While the composition of MT nucleation systems is to some extent heterogeneous across eukaryotic organisms, γ-tubulin, a member of the tubulin superfamily, is a universal determinant in this process. In Saccharomyces cerevisiae, Spindle Pole body Component 97 (Spc97) and Spc98 were identified to assemble with two molecules of yeast γ-tubulin (Tub4) into the 300-kDa heterotetrameric γ-tubulin small complex (γ-TuSC), forming the core of the MT nucleation system in lower eukaryotes. The γ-TuSC possesses a Y-like overall shape of 180 Å height and a width of 60-100 Å. It is composed of two interacting spokes, each comprising one copy of γ-tubulin and either one molecule of Spc97 or Spc98. The N-terminal GRIP1 domain mediates canonical interactions between the Spc subunits, while the C-terminal GRIP2 domain binds one copy of γ-tubulin.

We isolated recombinantly expressed C. albicans γ-TuSC from insect cells by affinity purification and anion-exchange chromatography and used cryo-EM single particle analysis to obtain a structure at near-atomic resolution. We thus divided the γ-TuSC into two individual segments, each comprising one Spc protein and one γ-tubulin molecule, and refined them separately. This approach increased global resolution to 3.6 Å and improved density quality towards the periphery of the complex. Visual inspection of overlap, cross-correlation between density segments, and root mean square deviation (R.M.S.D) of protein backbone atoms in the atomic models consistently indicate that both copies of γ-tubulin in our cryo-EM reconstruction adopt a ‘straight’ conformation, as typically observed for αβ-tubulin dimers in stable and ordered microtubules. Thus, γ-tubulins in the fungal γ-TuSC are in a conformation that can promote growth of ‘straight’ microtubule protofilaments without a conformational change. Our cryo-EM density of the C. albicans γ-TuSC indicates binding of GDP, rather than GTP, and it remains to be addressed whether a nucleotide exchange to GTP is required to promote microtubule nucleation activity as suggested by analysis of γ-tubulin mutants in S. cerevisiae. In C. albicans, the first cluster of interactions is mostly formed by hydrophobic interactions between the GRIP1 domains of Spc97 and Spc98. In particular, the long insertion in the Spc98 GRIP2 domain (Asn626-Leu656) is involved in extending the interface and bridges over the subunit interface to stably bind to the GRIP2 domain of Spc97. Similar as for the interface between the Spc97/98 GRIP1 domains, this interaction is stabilized by hydrophobic patches: Leu630, Leu631, Leu632, Phe636, Met637, and Leu639 of the Spc98 insertion are exposed to a hydrophobic binding pocket on the surface of Spc97. In C. albicans, the γ-tubulin arrangement strongly differs from MT symmetry, requiring γ-tubulin molecules to move 5 Å towards each other during activation.

>[2x]MPGETITLQVGQCGNQVGLQYWQQLATEHGIQSDGSSTPYPKDINDLQLQELNNSGSSPQSYPQQTKPNGKYRNDHPELFFTLSDSNTYTPRSILIDMEPSVIAKSTSALPMFNPRNVHLSNQGNGAANNWINGYKYGTEEEETLLNLIDREVDKCDNLSNFQLFHSVAGGTGSGVGSKMLEVISDRYGHKKLLNTFSIFPSNEDTSDVVVQPYNTILTLKRLIDYSDATFVFHNDSLNRIENILFNNNSNIQHDDNDLFLGANKLIALVSASVSNPLRFPGYMYSSMESIVSNLIPTPDLKFLTSSIAPFSTQKHNYLNEYDMLLELSNDRYKTNRVGGDTSYISMLNYLIGYNLDQREIRKGILKSQQRISFVPWVARSVLVVHGKKSPYLKNTNLEGIQVTNNTSMIDVFTKILKQFDLLIKRKAYLNRYYSSVEEENEVMEMFNESRESVKSIIDEYKACKEITYLDDDDEDDLEDGDGGGGGNGNGYNNIDDADMGI;> MNTFSSPPNVIREYNDSTYQSPLNSQFHQSPFLQTQSPDYVSLREEEDDNNDKNLDIMSSCIVDSVIYKSQKIAGPLLSQISNLNIQQALIIRELLFTLLGHEGHYIQYSKRYDPTSQISRIEGPDYKIAKNLDISLKVITKKLVKFGKFYSGLKSFIQVFDNNKFGKIVQKFCSEVRKFLSSYQQVLINVEHEFKFNKNFNLNMLDSLLHQEISNEMTHLYQIGIEISRITEERQKMSQAEIMGNFEPTTLANTSMNGINSEPNLYYGKFDCCKGGLLLQVIQERMVYYKGDPTSLDFLTQLFDIVSSDYIGMLNQWLLEGVINDPFDEFMIREKRVPDSFMEIFQSKSEYYWNELFLIKIDGLLNQFQNSTIQSKILNTGKYLNIFKRCTGLHNFESLKEKLTTITSLAAPDLELKIDEFYHRANKMLMKLLFDGYNFPSVVNIFQRLFLFADSFQIDNFIDSTFSELKRGKLKISVSRLQKQYDDIFKEKIENKVGVRPSVYDVLKKNQKLSVTSESLYKVVEELMEKNSDYLISDNNLRGIFHRVASLRDDSRLTISSTADSATENVKDEPTITSVDLTIPLPFPLNLVLNQQLSYQYEIMFKLLINIKFISKYNSSNWQEMNYSKIWTNSHFNSSVKKWILRCRVLHSRICSFIHELENYIVHDVIEHNFEEIKNLIHTTATNLATSELGSDINDEGDNIFNGSLIRGTFNNNSIFDSKVHKHRTTTYVEGISTVEQLIQKFLDYSSTLLNDSLLTREESLRQLRKMLDFIFHFNNYIVQVKKVLVLLNHELFNEYSKEFPTKFEKPMDQESIDKRFANLSDTFLMQYEKFGENLVTFLATIKQVGERENQGLLELSNRLELCFPE;> MALNKVQLIKLYSNRLVKSLVPVEFGEAFIQSIINDLQTTLLNTSSEEQNLSIIINKLKMQFLSNNLKNEWVEFQNIVNSLSKFKSLDQICNYLAFLDALRDEKPEDILSTSTASLSPGKQNLMINTVNTALTLSQLIEPYYDTLSEQTILTYLPYTMLGSDSKIFTFSNNYTRLEIPKDINNSFSSLLREVFEFAILYKQLAIVVDRYKGTLVSAIKTAYIAILEAQLNKYVNDINNIFNNKPNSILVVYNSIFPWISILRFLYRVSNRLNRLDGYEFLTFIYSFTNHGDPKIRGIAVTAFTEVVKPYYNIVEHWIVKGELIDNNNEFFIIFDQEQNEFNSIIKLLPKKIPAFIKSSDKIFQIGKTLIFLNKYCRELKWVNQYNVKYSAILFNNHQGLASMTTNEMIKLIDSQYNEILTFLTQIIQGNNKLFTHVYNFKRFYFMETNDFIDAIMVKGKDVFNESSVNISSTYLRKVLQDAIQISSVKNFEYVDRLDSRVLNPQHGNLGWESFTIEYKIDDLPMSYLFEGHQHLQYLKMFHFLWKLRQLNNLLNWHFEMFNELNHNVVTKLSSRNRRPLAKSLSIITSIRFHFTQFLNELIAYLSYDVIEENFQQHIVRKLFYNKNDQDLLLNKSFMNLSEIDPNNDLPKFNVNLLTIDELVELHGTYIDSIINSSLLNEKLKGNETNISYIDQIFNILQTIFNFINTSQEFYSLVVTFGLLVRSDSNANKIELEQDQEDLEFQLHKIKRKIYKDIYQHDYKRQLNDLKNDLNRDYNLKDLSKLL> XXXXXXXXXXXXXXXXXXXXXXXXXXXFRKLLYKLDLRLFQTISDQMTRDLKDILDINVSNNELCYQLKQVLARKEDLNQQIISVRNEIQELKAGKDWHDLQNEQAKLNDKVKLNKRLNDLTSTLLGKYEGDRKIMSQDSEDDSIRDDSNIL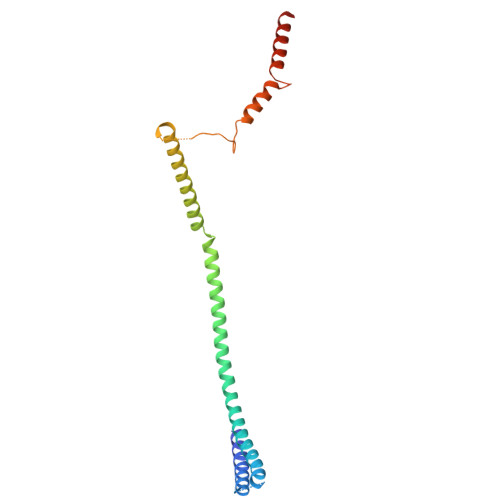DIAHFVDLMDPYNGLLKKINKINENLSNELQPSL>GPHMTELLFNKRLQVLVKSKDTDERRSVIRVSIELQLPSSPVHRKDLVV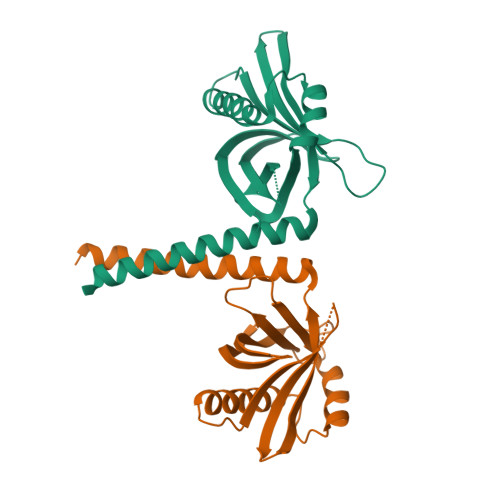RLTDDTDLYFLYNLIISEEDFQSLKVQQGLLIDFTSFPQKFIDLLEQCICEQDKENPRFLLQLSSSSSAFDHSPSNLNIVETNADKHLTHLSLKLLPGSDTDIKKYLASCLSSVKEEKQQLQQKLRKTEEDLT[3x]N-hydroxy-4-[5-(morpholin-4-yl)-7-oxo-7H-thieno[3,2-b]pyran-3-yl]benzamide | C18 H16 N2 O5 S | 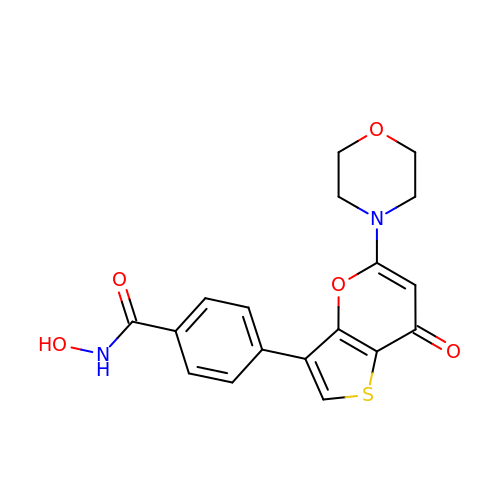SEKOPSVILCFYRX-UHFFFAOYSA-N hydrogen arsenate | As H O4 | 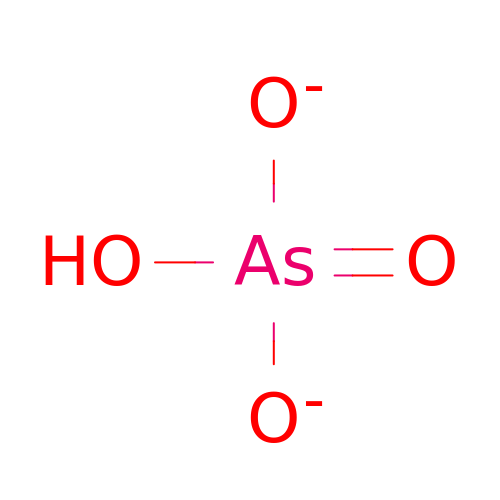DJHGAFSJWGLOIV-UHFFFAOYSA-L> AEGSQACAKGCELCSEVNGCLKCSPKLFILLE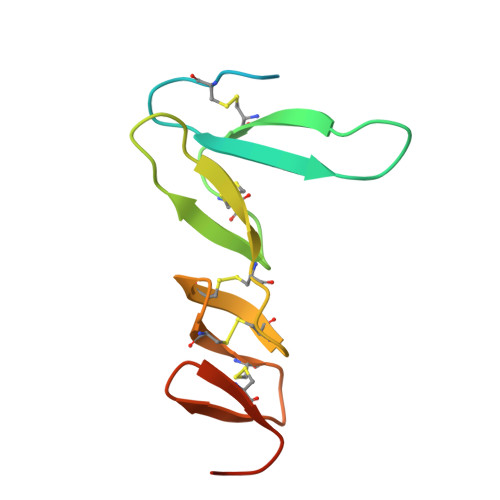RNDIRQVGVCLPSCPPGYFDARNPDMNKCIKCKIEHCEACFSHNFCTKCKEGLYLHKGRCYPACPEGSSA> XXXXXXXXXXXXXXXSILRLLETNTVSALDSVFEKYEKEMNQMTHGDNNEVKRIYSKKERLLEIILTKIKKKLRQAKFPSRISERDLDIEYIYSKRQFIQNRYSQELQNNERLEAILSREQNLLEETRKLCMNLKTNNKKRLTEKLIQKDLHPVLNKAMEYTYGLESTNGFMHPDGPVTFRNDSHELNLMLNDPIKSTADVRLDKEEVLSLLPSLKEYTKKSKE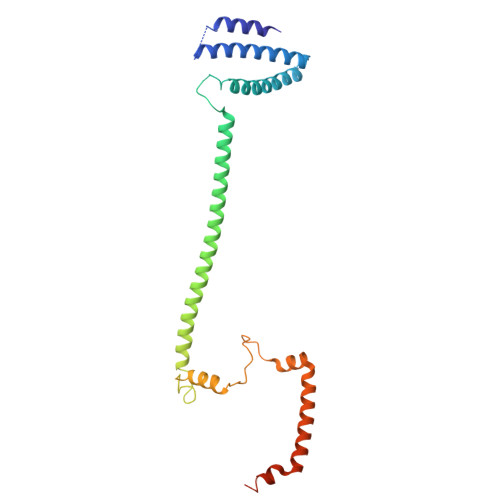LKETMGQMISDSHEEEIKEVFVPHHESHQDKTEEDIH>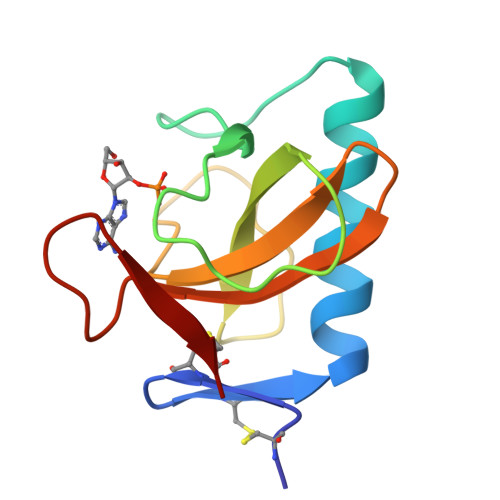 ACDYTCGSNCYSSSDVSTAQAAGYKLHEDGETVGSNSYPHKYNNYQGFDFSVSSPYYEWPILSSGDVYSGGSPGADRVVFNENNQLAGVITHTGASGNNFVECT> MEKQGEKMKRL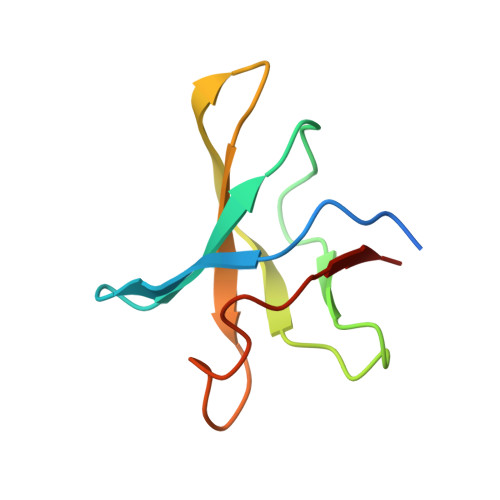GKVLHYAKQGFLIVRTNWVPSLNDRVVDKRLQFVGIVKDVFGPVKMPYVAIKPKVSNPEIYVGEVLYVDER N-hydroxy-5'-O-(2-methylpropanoyl)cytidine 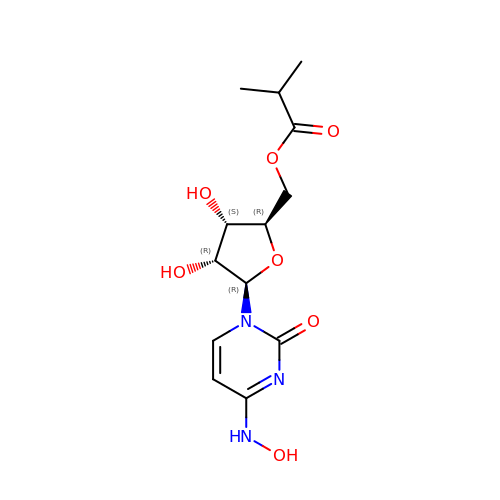| C13 H19 N3 O7 | HTNPEHXGEKVIHG-QCNRFFRDSA-N>[2x]MDICWNSPLFLVCVV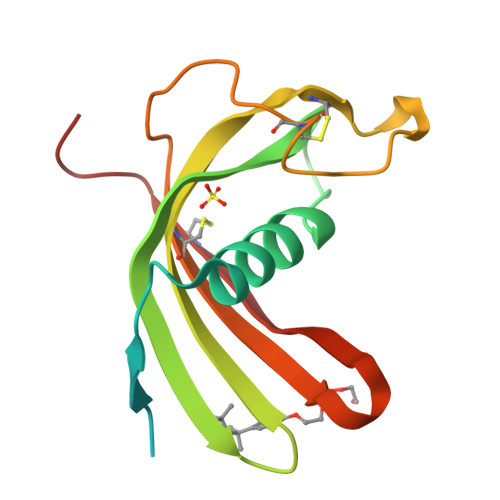LAAAGSASRSKRALVGGWKTQDPTNPKFENLAHYAVSTQVEGREYYDTVLELLEVQTQIVAGVNYKLKFTTTQSTCKIESGVEYSKELCQPKTNKVEAVCTSIIYTVPWQNIKRVLSYHCDAPNNV> GDRVADVIESSIGDSVSRALTRALPAPTGQDTQVSSHRLDTGKVPALQAAEIGASSNASDESMIETRCVLNSHSTAETTLDSFFSRAGLVGEIDLPLEG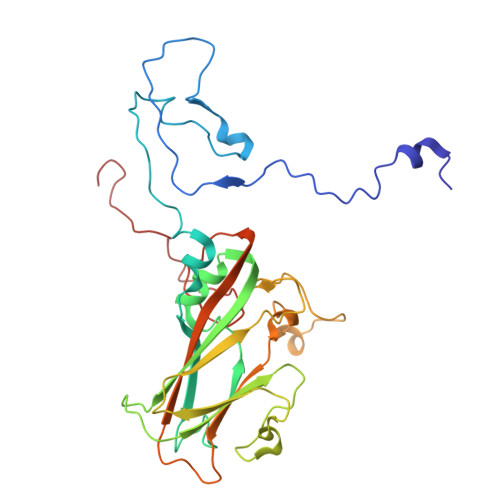TTNPNGYANWDIDITGYAQMRRKVELFTYMRFDAEFTFVACTPTGQVVPQLLQYMFVPPGAPKPDSRESLAWQTATNPSVFVKLSDPPAQVSVPFMSPASAYQWFYDGYPTFGEHKQEKDLEYGACPNNMMGTFSVRTVGTSKSKYPLVIRIYMRMKHVRAWIPRPMRNQNYLFKANPNYAGNFIKPTGASRTAITTL> MYLTKEEELILAGEYGYALQKAMEILVALGDIYGADRLIPIKSAQVAGVSYKNIGDAGIEFLRDFVEAGAKVSVYTTLNPAGIGDDEFMEKQME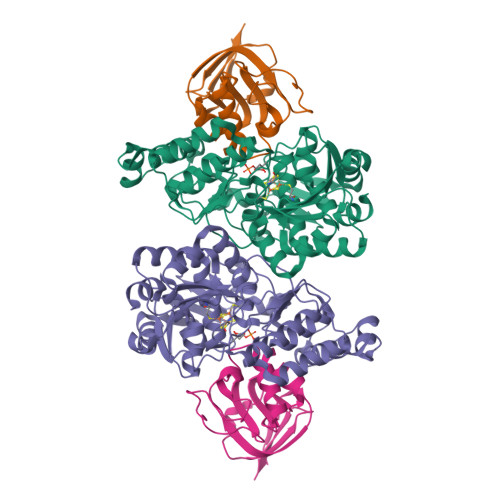VLELYRKMGIEVTSTCTPYYGANLPKFGDHIAWSESSAVSFANSILGARTNREGGPSSLAAAIVGKTPNYGLHLDENRKATVIVDVKAKVKTFADYSVLGYHVGKTLGNDVPYFKNLKPEKTEFLKELGAAMGATGSIALYHVEGETPEYREAITDKLETITVEDSDLKAVRESFQDDWSDIDMILIGCPHASLPEVKEIAELLRMRGKPLKIPLFITASRAVKALADALGYTEIIERYNGKIIPDSCFVVSPIKGWYRGIATNSGKSAFYFRSFGFSVRLDDVENLIKEAP;> GPKLKGRKIVGGKAEGEVIVSRKPLSFLGGVDPETGIVTDAESDIRGQSIAGKILVFPRGKGSTVGSYVIYALKKNNKAPKAIIVGEAETIVATGAIISDIPMVDGVDVSKLKTGMKVRVDADSGEVEILEDGE>[2x]MEDMILTEEMQKIMNLIQDDENNVFVTGKAGSGKTTFLKYLIEKSGKNCIVAAPTGIAAINAGGVTLHSLFGIPFGPITPYDRLENKFSEYKVELLLKMELLIIDEISMVRPDILDTIDRKLRWVYESDEPFGGVQVVMFGDLFQLPPVTKKQEREILSDFYDGFFFFNALVFKRTGFHIVELTKIFRQTEPEFINVLNNIRNYQVTSDELDLLSELKDRKISSSYDNEYIHICTHKADVEKINADKLGEQEIRNYDIVIKDKFPESSIPCDLHLKLRVGARVMSLVNDSLKGYYNGMLGIVTALEDNVITVRMDNGRTIKFERYTWSNTQYTLKDNEIVKEEIGSCTQFPLTLAWAITIHKSQGLTFDKIIIHVSHTFCPGQLYVALSRCRTLEGIVSDAFITKQMIIPEYALIDFERAYKSEGNYYGKRLD

Helicases are modular motor proteins that couple the binding and hydrolysis of ATP to unwinding of double-stranded (ds) DNA and play essential roles in nearly all aspects of nucleic acid metabolism, ranging from DNA replication to chromatin remodeling. Pif1 is evolutionarily conserved from bacteria to humans. Pif1 unwinds duplex DNA in a single-base-pair kinetic step, powered by the hydrolysis of one ATP molecule. To reveal the structural basis for unwinding dsDNA by Pif1, we determined the structure of BaPif1 in complex with a symmetrical dual forked dsDNA and ADP·AlF4−.

We crystallized BaPif1 in complex with ADP·AlF4– and a symmetrical dual forked dsDNA containing a 10 nt oligo-dT at both 3′ and 5′ ends (designated as BaPif1–10dT-fdsDNA) and determined its structure at a resolution of 3.3 Å. The asymmetric unit of the crystal structure contains two BaPif1 molecules plus one DNA strand, thus the model of the biologically meaningful BaPif1–10dT-fdsDNA complex is generated by the application of a crystallographic two-fold operation. The structure of BaPif1–10dT-fdsDNA showed that two BaPif1 molecules bind to each fork of 10dT-dsDNA and interact with their respective forks in the same manner. The two BaPif1 molecules bound to the junction regions of one fork are related by a rotation of 68° rather than 180°. The binding of BaPif1 to the 5′ arm causes a sharp bend between T10 and C11; consequently, the base of T10 points in the direction opposite to those of other oligo-dTs. The flipped base of T10 is sandwiched between Tyr91A and Tyr412B. Importantly, the bending in the 5′ ss/dsDNA junction breaks the first C11–G20 base-pair. Another notable feature is that three residues His236B, His377B and Phe379B from BaPif1 bound to the 3′ ss/dsDNA are juxtaposed at the helical junction of ss/dsDNA junction. BaPif1 bound to the 5′ arm uses loops β11–β12, β12–β13 and β14 of the 2B domain to interact with loop α8–α9, helices α9 and α13 of the 2A domain in the BaPif1 bound to the 3′ ss/dsDNA junction predominantly through a network of salt bridge contacts and hydrogen bonds. First, the BaPif1 molecule bound to the 5′ arm initiates the forked DNA unwinding by breaking the first base-pair through geometrical strain while the BaPif1 molecule bound to the 3′ arm plays an accessory role in unwinding through stabilizing the first broken base-pair and engaging the second base-pair in a pre-breaking state.> MKLALLASLVASAAAFAPSKVAQTSTALKAFENELGAQPPLGFFDPLGLVEDGNQAKFDRLRYVELKHGRISMLAVVGYLIEKAGIRLPGNISYDGTSFADIPDGFAALSKIPDAGLFQLFAFIGFLEVFVMKDITGGEFVG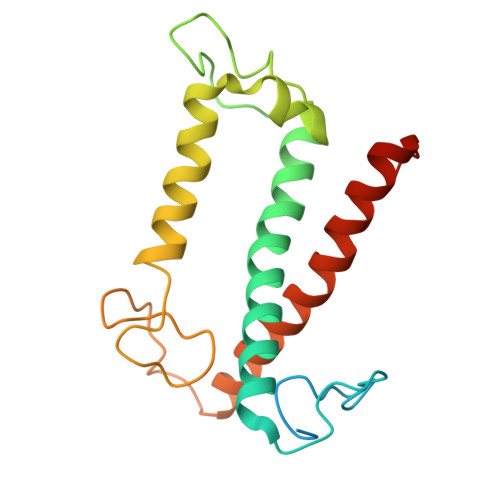DFRNGFIDFGWDSFDEETKLKKRAIELNQGRAAMMGILALMVHEKLGVSLLPQ>[2x]ASRNQSSCDTVDQG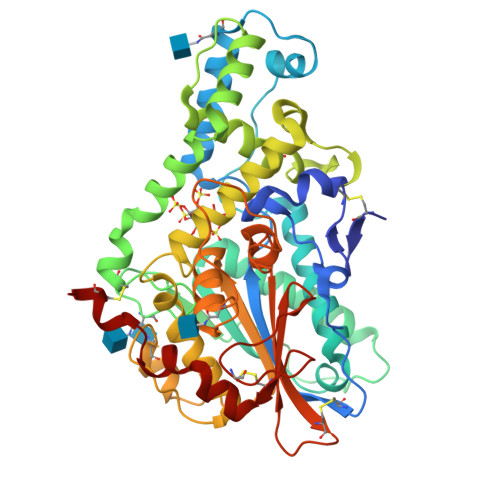YQCFSETSHLWGQYAPFFSLANESVISPEVPAGCRVTFAQVLSRHGARYPTDSKGKKYSALIEEIQQNATTFDGKYAFLKTYNYSLGADDLTPFGEQELVNSGIKFYQRYESLTRNIVPFIRSSGSSRVIASGKKFIEGFQSTKLKDPRAQPGQSSPKIDVVISEASSSNNTLDPGTCTVFEDSELADTVEANFTATFVPSIRQRLENDLSGVTLTDTEVTYLMDMCSFDTISTSTVDTKLSPFCDLFTHDEWINYDYLQSLKKYYGHGAGNPLGPTQGVGYANELIARLTHSPVHDDTSSNHTLDSSPATFPLNSTLYADFSHDNGIISILFALGLYNGTKPLSTTTVENITQTDGFSSAWTVPFASRLYVEMMQCQAEQEPLVRVLVNDRVVPLHGCPVDALGRCTRDSFVRGLSFARSGGDWAECFA> MSQSNRELVVDFLSYKLSQKGYSWSQFSDVEENRTEAPEETEAERETPSAINGNPSWHLADSPAVNGATGHSSSLDAREVIPMAAVKQALREAGDEFELRYRRAFSDLTSQLHITPGTAYQSFEQVVNELFRDGVNWGRIVAFFSFGGALCVESVDKEMQVLVSRIASWMATYLNDHLEPWIQENGGWDTFVDLYGNNAAAESRKGQERFN;> APPNLWAAQRYGRELRRMSDEFEGSFK

The BCL-2 family proteins, which are commonly known as positive or negative regulators of apoptosis, are characterized as containing up to four conserved stretches of amino acids, known as BCL-2 homology (BH) domains. The interactions between such proapoptotic BCL-2 family members and the antiapoptotic members, such as BCL-2 and BCL-XL, are the crucial events in controlling or promoting apoptosis. These interactions are mediated by the BH3 domain of the proapoptotic members that binds to a site known as the BH3-binding groove in the antiapoptotic members. In addition to their critical roles in the regulation of apoptosis, the BCL-2 family proteins have emerged as regulators of autophagy, a catabolic process that plays crucial roles in cell survival, tumor suppression, and innate immune defense against intracellular pathogens by degrading cytoplasmic components through lysosomal pathway.

For a detailed structural comparison, we used the crystal structure of BCL-XL in complex with BAD that we have determined to 2.3 Å resolution, in which 27 residues of BAD bound to BCL-XL as an extended α-helix and all the rest of the residues were totally disordered. A sequence alignment based on the structural comparison showed that four out of five residues within proapoptotic BH3 domains that are critical for their interactions with the BH3-binding groove are conserved as Leu110, Leu114, Asp119 and Phe121 in Beclin1. The remaining residue, which is isoleucine or methionine in the BH3 domains, is substituted as Thr117 in Beclin1. These five residues occupy spatially and chemically equivalent positions at the BH3-binding groove of M11 as the corresponding residues of BAD bound to BCL-XL. Another noticeable difference from the canonical BH3 domains is that the Beclin1 α-helix has a hydrophobic patch composed of Val116, Leu120 and Ile123 that are not shielded by the BH3-binding groove, while those of other BH3 domains, including that of BAD, are distinctively amphipathic. The Beclin1 helix has a hydrophobic patch (indicated by an asterisk) on the opposite side of the BH3-binding groove, unlike the BAD helix.>MRYFYDTEFIEDGHTIELISIGVVAEDGREYYAVSTEFDPERAGSWVRTHVLPKLPPPASQLWRSRQQIRLDLEEFLRIDGTDSIELWAWVGAYDHVALCQLWGPMTALPPTVPRFTRELRQLWEDRGCPRMPPRPRDVHD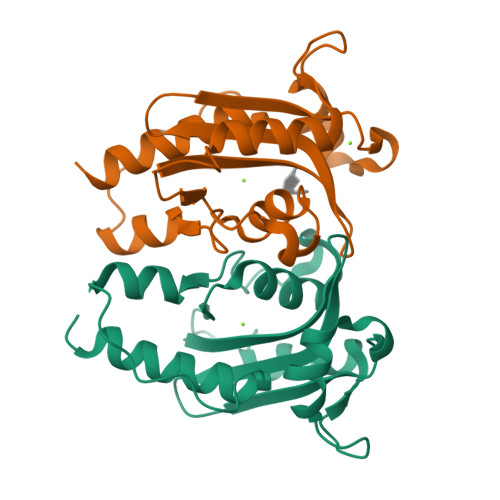ALVDARDQLRRFRLITSTDDAGRGAAR[2x]>[12x]RTGLAEDGAKSVYERLKNDRAPYETRAQNCAQYTIPSLFPKDSDNASTDYQTPWQAVGARGLNNLASKLMLALFPMQTWMRLTISEYEAKQLLSDPDGLAKVDEGLSMVERIIMNYIESNSYRVTLFEALKQLVVAGNVLLYLPEPEGSNYNPMKLYRLSSYVVQRDAFGNVLQMVTRDQIAFGALPEDIRKAVEGQGGEKKADETIDVYTHIYLDEDSGEYLRYEEVEGMEVQGSDGTYPKE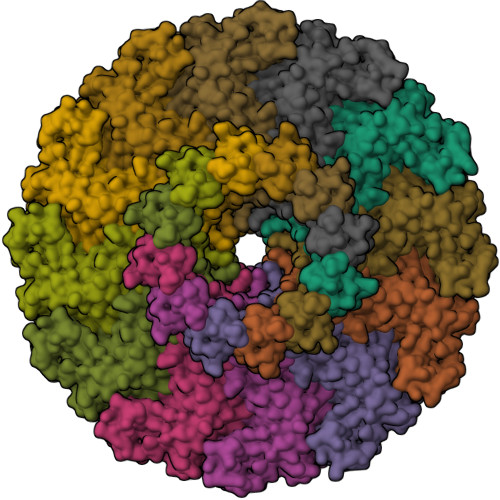ACPYIPIRMVRLDGESYGRSYIEEYLGDLRSLENLQEAIVKMSMISSKVIGLVNPAGITQPRRLTKAQTGDFVTGRPEDISFLQLEKQADFTVAKAVSDAIEARLSFAFMLNSAVQRTGERVTAEEIRYVASELEDTLGGVYSILSQELQLPLVRVLLKQLQATQQIPELPKEAVEPTISTGLEAIGRGQDLDKLERCVTAWAALAPMRDDPDINLAMIKLRIANAIGIDTSGILLTEEQKQQKMAQ S-bicalutamide | C18 H14 F4 N2 O4 S | 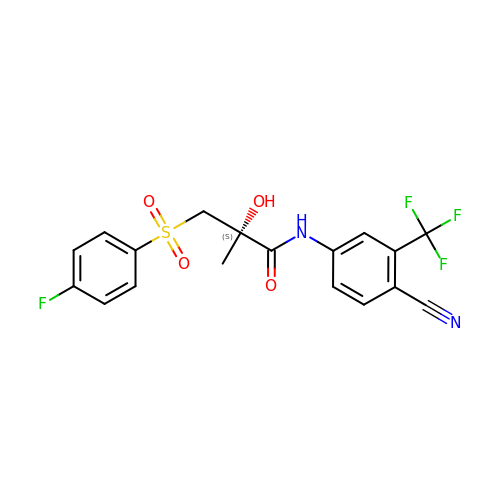LKJPYSCBVHEWIU-QGZVFWFLSA-N>SGRPSTDALKLCPHEEFLRLCKERAEEIYPIKERNNRTRLALIICNTEFDHLPPRNGADFDITGMKELLEGLDYSVDVEENLTA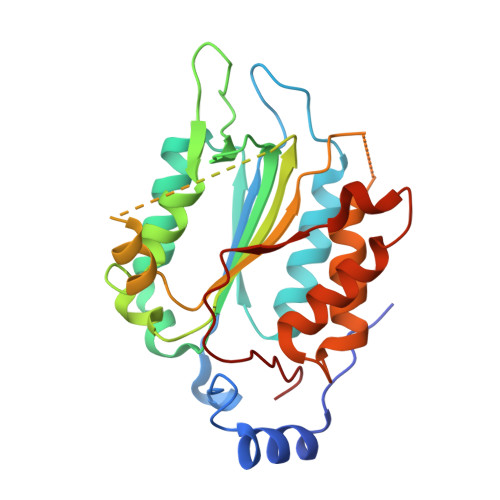RDMESALRAFATRPEHKSSDSTFLVLMSHGILEGICGTVHDEKKPDVLLYDTIFQIFNNRNCLSLKDKPKVIIVQAARGANRGELWVRDSPASLEVASSQSSENLEEDAVYKTHVEKDFIAFCSSTPHNVSWRDSTMGSIFITQLITCFQKYSWCCHLEEVFRKVQQSFETPRAKAQMPTIERLSMTRYFYLFPGN[2x];>[2x]GPLGSGRPMLSTDNFKKIKLRDISLEDAIKASNYEEINNKVTDKKMAHQALAYSLGNKKADIALYLLSKFNFTKQDVAEMEKMKNNRYCNLYDVEYLLSKDGANYKVLEYFINNGLVDVNKKFQKVNSGDTMLDNAMKSKDSKMIDFLLKNGAILGKRFEI>MAEKNYVMAIDQGTTSSRAIIFDRNGKKIGSSQKEFPQYFPKSGWVEHNANEIWNSVQSVIAGAFIESGIRPEAIAGIGITNQRETTVVWDKTTGQPIANAIVWQSRQSSPIADQLKVDGHTEMIHEKTGLVIDAYFSATKVRWLLDNIEGAQEKADNGELLFGTIDSWLVWKLTDGQVHVTDYSNASRTMLYNIHKLEWDQEILDLLNIPSSMLPEVKSNSEVYGHTRSYRFYGSEVPIAGMAGDQQAALFGQMAFEKGMIKNTYGTGAFIVMNTGEEPQLSDNDLLTTIGYGING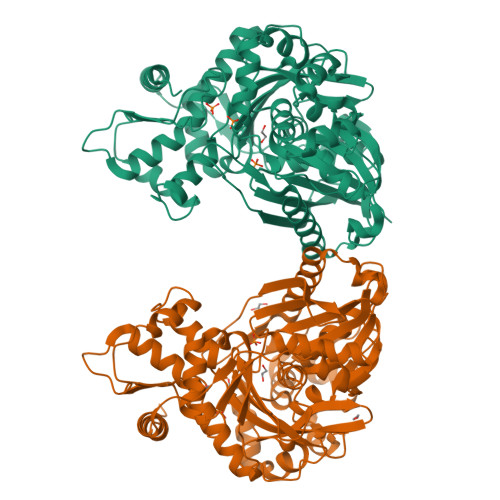KVYYALEGSIFVAGSAIQWLRDGLRMIETSPQSEELAAKAKGDNEVYVVPAFTGLGAPYWDSEARGAVFGLTRGTTKEDFVRATLQAVAYQSKDVIDTMKKDSGIDIPLLKVDGGAAKNDLLMQFQADILDIDVQRAANLETTALGAAYLAGLAVGFWKDLDELKSMAEEGQMFTPEMPAEERDNLYEGWKQAVAATQTFKFKAKKEGE[4x]>SVRRDRAPPERGGAGTSQDGTSKNWFKITIPYGRKYDKAWLLSMIQSKCSVPFTPIEFHYENTRAQFFVEDASTASALKAVNYKILDRENRRISIIINSSAPPHTILNELKPEQVEQLKLIMSKRYDGSQQALDLKGLRSDPDLVAQNIDVVLNRRSCMAATLRIIEENIPELLSLNLSNNRLYRLDDMSSIVQKAPNLKILNLSGNELKSERELDKIKGLKLEELWLDGNSLCDTFRDQSTYISAIRERFPKLLRLDGHELPPPIAFDVEAPTTLPPCKGSYFGTENLKSLVLHFLQQYYAIYDSGDRQGLLDAYHDGACCSL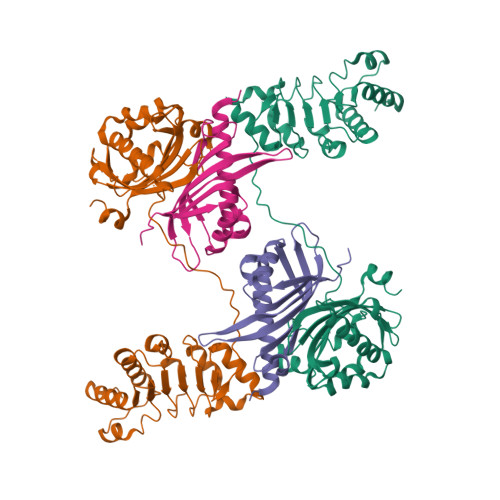SIPFIPQNPARSSLAEYFKDSRNVKKLKDPTLRFRLLKHTRLNVVAFLNELPKTQHDVNSFVVDISAQTSTLLCFSVNGVFKEVDGKSRDSLRAFTRTFIAVPASNSGLCIVNDELFVRNASSEEIQRAFAMPAPTP[2x];>ASVDFKTYVDQACRAAEEFVNVYYTTMDKRRRLLSRLYMGTATLVWNGNAVSGQESLSEFFEMLPSSEFQISVVDCQPVHDEATPSQTTVLVVICGSVKFEGNKQRDFNQNFILTAQASPSNTVWKIASDCFRFQDWAS[2x]> SLTPLSAITVRSMEGPPTVQQQSPSVIRQSPTQRRKTSTTSSTSRAPPPTNPDASSSSSSFAVPTIHFKESPFYKIQRLIPELVMNVEVTGGRGMCSAKFKLSKADYNLLSNPNSKHRLYLFSGMINPLGSRGNEPIQFPFPNELRCNNVQIKDNIRGFKSKPGTAKPADLTPHLKPYTQQNNVELIYAFTTKEYKLFGYIVEMITPEQLLEKVLQHPKIIKQATLLYLKKTLREDEEMGLTTTSTIMSLQCPISYTRMKYPSKSINCKHLQCFDALWFLHSQLQIPTWQCPV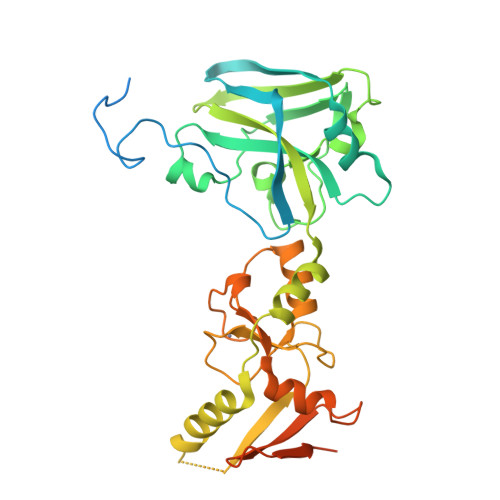CQIDIALENLAISEFVDDILQNCQKNVEQVELTSDGKWTAILEDDDDSDSDSNDGSRSPEKGTLGEGAAALEHHHHHH ETHANEPEROXOIC ACID | C2 H4 O3 | 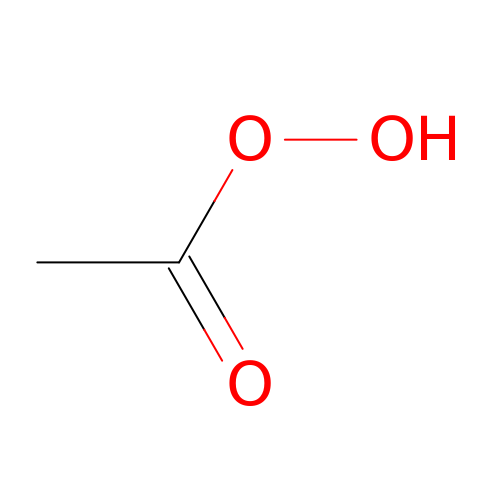KFSLWBXXFJQRDL-UHFFFAOYSA-N> MWRLSRVALQSNRAALYMPYTPVATNPVVYFDITAEGDALGRVSVELFRDVVPRTSENFRSLCTGERGYGQCLLYYKGTPFHRIIPGFVMQGGDILTKDGRSNVSVFGYPFPDESFEGKAGKHLPGTVGMAHSGPNQNGSQFFFNLGRNEQLDRKFVVVGQVLGGWEIVNQVVKLCGSRCGTPVSRAWISDCGQ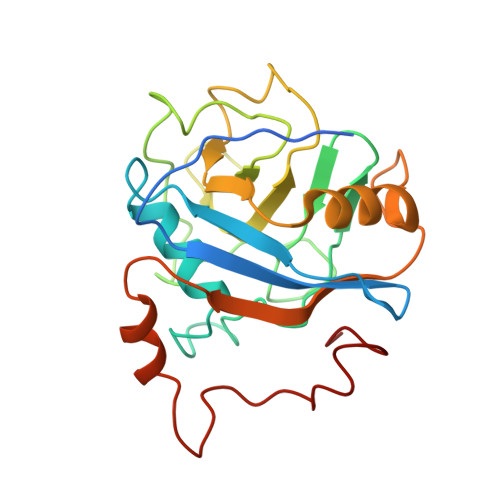SGGYMAEETQEALQGERAQHVIPGKEVLDLIQPRY>SEEVVIAGMSGKLPESENLQEFWANLIGGVDMVTDDDRRWKAGLYGLPKRSGKLKDLSKFDASFFGVHPKQAHTMDPQLRLLLEVSYEAIVDGGINPASLRGTNTGVWVGVSGSEASEALSRDPETLLGYSMVGCQRAMMANRLSFFFDFKGPSIALDTACSSSLLALQNAYQAIRSGECPAALVGGINLLLKPNTSVQFMKLGMLSPDGTCRSFDDSGSGYCRSEAVVAVLLTKKSLARRVYATILNAGTNTDGSKEQGVTFPSGEVQEQLICSLYQPAGLAPESLEYIEAHGTGTKVGDPQELNGITRSLCAFRQAPLLIGSTKSNMGHPEPASGLAALTKVLLSLEHGVWAPNLHFHNPNPEIPALLDGRLQVVDRPLPVRGGNVGINSFGFGGSNVHVILQPNTRQAPAPTAHAALPHLLHASGRTLEAVQDLLEQGRQHSQDLAFVSMLNDIAATPTAAMPFRGYTVLGVEGRVQEVQQVSTNKRPLWFICSGMGTQWRGMGLSLMRLDSFRESILRSDEAVKPLGVKVSDLLLSTDERTFDDIVHAFVSLTAIQIALIDLLTSVGLKPDGIIGHSLGEVACGYADGCLSQREAVLAAYWRGQCIKDAHLPPGSMAAVGLSWEECKQRCPAGVVPACHNSEDTVTISGPQAAVNEFVEQLKQEGVFAKEVRTGGLAFHSYFMEGIAPTLLQALKKVIREPRPRSARWLSTSIPEAQWQSSLARTSSAEYNVNNLVSPVLFQEALWHIPEHAVVLEIAPHALLQAVLKRGVKSSCTIIPLMKRDHKDNLEFFLTNLGKVHLTGINVNPNALFPPVEFPAPRGTPLISPHIKWDHSQTWDVPVAEDFPN[4x]

De novo fatty acid biosynthesis in humans is accomplished by a multidomain protein, the Type I fatty acid synthase (FAS). However, FAS is overexpressed in cancer cells and correlates with tumor malignancy, which makes FAS an attractive selective therapeutic target in tumorigenesis.

Herein, we present a crystal structure of the condensing part of murine FAS, highly homologous to human FAS, with octanoyl moieties covalently bound to the transferase (MAT—malonyl‐/acetyltransferase) and the condensation (KS—β‐ketoacyl synthase) domain. The MAT domain binds the octanoyl moiety in a novel (unique) conformation, which reflects the pronounced conformational dynamics of the substrate‐binding site responsible for the MAT substrate promiscuity. In contrast, the KS binding pocket just subtly adapts to the octanoyl moiety upon substrate binding. Besides the rigid domain structure, we found a positive cooperative effect in the substrate binding of the KS domain by a comprehensive enzyme kinetic study. These structural and mechanistic findings contribute significantly to our understanding of the mode of action of FAS and may guide future rational inhibitor designs.> ACGTCA;> GAACGACAGTGACGTCGACTC;> TCGAGTCG;> CTGTCGT

In this work, we exhaustively probe the ability of all 36 immobile HJ sequences to form DNA crystals in two different designed systems. Three separate self-assembling DNA crystal systems are described in this report: the “4 × 5” and “4 × 6” designs (collectively referred to as the 4 × N systems), and a third construct with a “scrambled” sequence variant of the 4 × 6 lattices. Self-assembly was mediated by three constituent oligonucleotides: (S1) containing four sequence repeats of either 5 or 6 bases; (S2) composed of 21 bases containing complementary regions to both (S1); and (S3) which forms the second junction crossover. The HJ serves as the fundamental component at the core of each unit, and the ultimate assembly of the full lattice is facilitated by the complementary 2-base sticky ends that tail each duplex.

Each asymmetric unit could be defined as either a HJ containing 10 and 11 bp on each arm, or as a 21-bp linear duplex. To investigate this possibility, we designed “scrambled” sequences with targeted base substitutions, while maintaining GC content, along each “stem”. Contrary to the buffer preference observed with the native P32 crystals, the scrambled systems exhibited an exclusive preference towards low salt buffers, much like the native R3 crystals. Remarkably, only J1 and J2 retained the P32 symmetry, with all others yielding an R3 lattice. There appeared to be only a marginal difference in the average cell lengths in the R3 scramble crystals (a = b = 113.04 c = 51.10) relative to the native 4 × 6 sequences: the a, b axis trended ~2 Å shorter and c ~1.3 Å longer, whereas in the J1 and J2 cases, the crystals were in good agreement with the original 4 × 6 motif. The average angles of the R3 and P32 crystals were 61.00° (σ = 1.21) and 58.05° (σ = 1.39), respectively. However, in the majority of the crystal structures reported here, the cacodylate anion indeed fits best into the electron density map of our X-ray structures, due to the presence of sodium cacodylate in the crystallization solution.>[2x]GAMEMNMADAPLEEGLLVCTRLDQNLCAELISFGSGKATVCLTPKEFMLCEDDVVHAGFIVGAASFAALC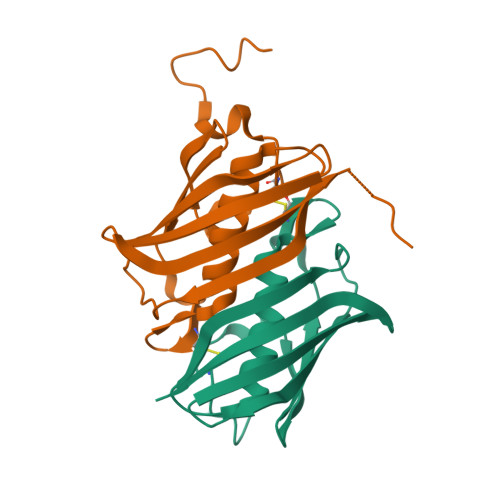ALNKKNSLISSMKVNLLAPIEIKQEIYFNATITHTSSKKSTIRVEGEFMEIKVFEGDFEILVFEKRPFKFNFKED>[2x]APRKFFVGGN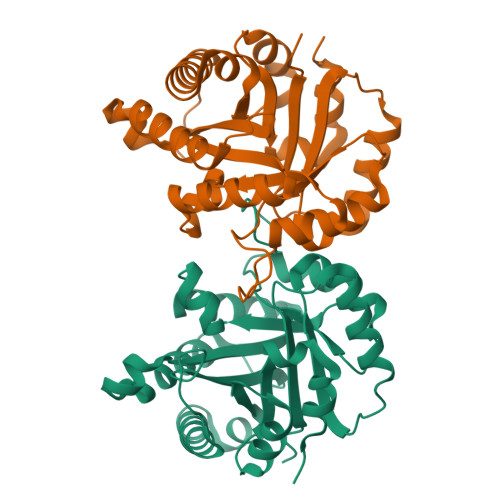WKMNGKRKSLGELIHTLDGAKLSADTEVVCGAPSIYLDFARQKLDAKIGVAAQNCYKVPKGAFTGEISPAMIKDIGAAWVILGHSERRHVFGESDELIGQKVAHALAEGLGVIACIGEKLDEREAGITEKVVFQETKAIADNVKDWSKVVLAYEPVWAIGTGKTATPQQAQEVHEKLRGWLKTHVSDAVAVQSRIIYGGSVTGGNCKELASQHDVDGFLVGGASLKPEFVDIINAKH> GSNIESTLNSVASVKDLANEASKYEIILQKGINQVGLKQYTQVVHKLDDMLEDIQSGQANREENSEFHGILTHLEQLIKRSEAQLRVYFISILNSIKPFDPQINITKKMPFPYYEDQQLGALSWILDYFHGNSEGSIIQDILVGERSKLILKCMAFLEPFAKEISTAKNAPYEKGSSGMNSYTEALLGFIANEKSLVDDLYSQYTESKPHVLSQILSPLISAYAKLFGANLKIVRSNLENFGFFSFELVESINDVKKSLRGKELQNYNLLQDCTQEVRQVTQSLFRDAIDRIIKKANSISTIPSNNGVTEATVDTMSRLRKFSEYKNGCLGA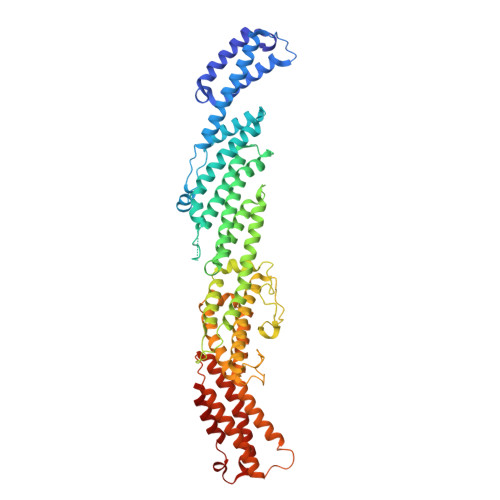MDNITRENWLPSNYKEKEYTLQNEALNWEDHNVLLSCFISDCIDTLAVNLERKAQIALMPNQEPDVANPNSSKNKHKQRIGFFILMNLTLVEQIVEKSELNLMLAGEGHSRLERLKKRYISYMVSDWRDLTANLMDSVFIDSSGKKSKDKEQIKEKFRKFNEGFEDLVSKTKQYKLSDPSLKVTLKSEIISLVMPMYERFYSRYKDSFKNPRKHIKYTPDELTTVLNQLVR>HHHHHHMATLKRDKGLDNTLKVLKQGYLYTTNQRNRLNTSVFQTKALGGKPFVVVTGKEGAEMFYNNDVVQREGMLPKRIVNTLAGKGAIHTVDGKKHVDRKALFMSLMTEGNLNYVRELTRTLWHANTQRMESMDEVNIYRESIVLLTKVGTRWAGVQAPPEDIERIATDMDIMIDSFRALGGAFKGYKASKEARRRVEDWLEEQIIETRKGNIHPPEGTALYEFAHWEDYLGNPMDSRTCAIDLMNTFRPLIAINRFVSFGLHAMNENPITREKIKSEPDYAYKFAQEVRRYY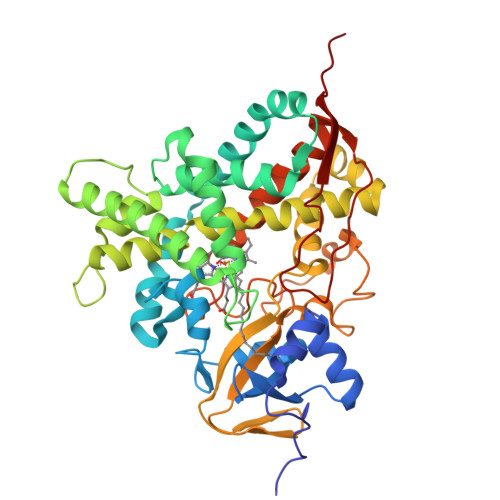PFVPFLPGKAKVDIDFQGVTIPAGVGLALDVYGTTHDESLWDDPNEFRPERFETWDGSPFDLIPQGGGDYWTNHRCAGEWITVIIMEETMKYFAEKITYDVPEQDLEVDLNSIPGYVKSGFVIKNVREVVDRT[2x]> MVKYPKQLFLESKNSKMNSIEMKYGQDPAINRAEFHVYGGVRQSKRKSEAWEAAKRITKERGIPNYNPDLHLKGAQMGQKVLQTYRITGLDREWAGGEDTPAHKGWKPGTDIAGLEMDDLNYENNPAMQQCYDDMRRTAINGLSIAHETIERRFGKEVTPETINLYFEMLNHNIGAGAIMMEHTAETNPELVKDSYAKCFTGNDELADALDQRFLIDINKMFPKYQADQIKAEVGDRIFQVARIPTMAVRTSDGGLSRAWVGQQASLAFLCAYDIPAGDAVTSDFVFTIKHGDVVFMGTQLPYRRAQRNNSAGGIALGYYSDCNQTSRTPEALEGLDGGIDPVKVIVEALTP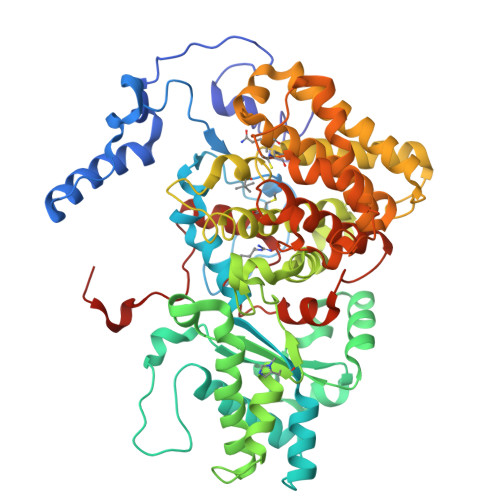GCVITDQGWLHNYLAGGSSGWSNYIISVYTDEVLEDYGYHGAIYAMDKWKCGVGEVPNTYENMMTIAEEVSRWSQKNYDEYPGLMEAHFGGSQRYSIQAAASGAAVGAMTGDPDLGNAAWHYNTPLCKEHYLRLGFYGHDLQDQQNMGHTYSYRSDQGIPYELKGPNYPDFAMNVGHMGGYIGIIAGAAHARGAAYSTNPIIKAAFADPNLQFDFRYPRREFGIGGLRQFMPAGERDAVIPPH>SHMAGLEVLFASAAPAITCRQDALVCFLHWEVVTHGYCGLGVGDQPGPNDKKSELLPAGWNNNKDLYVLRYEYKDGSRKLLVKAITVESSMILNVLEYG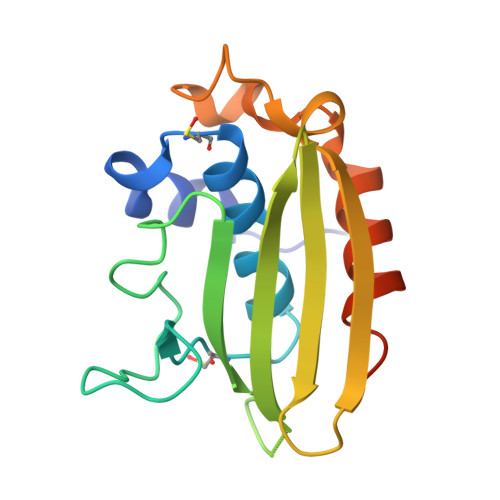SQQVADLTLNLDDYIDAEHLGDFHRTYKNSEELRSRIVSGIITPIHEQWEKANV[2x]>CGGAAA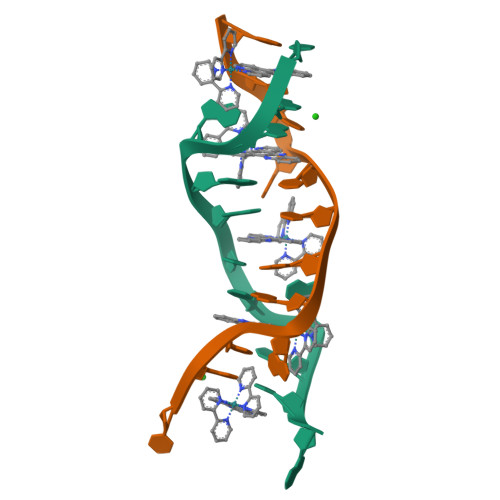TTACCG[2x]>[4x]MDIKINDITLG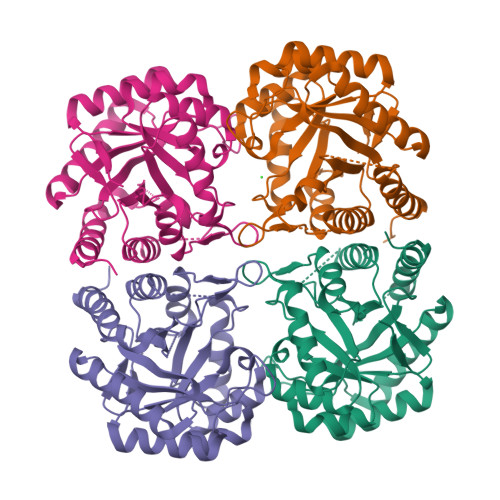NNSPFVLFGGINVLESLDSTLQTCAHYVEVTRKLGIPYIFKASFDKANRSSIHSYRGVGLEEGLKIFEKVKAEFGIPVITDVHEPHQCQPVAEVCDVIQLPAFLARQTDLVVAMAKTGNVVNIKKPQGLSPSQMKNIVEKFHEAGNGKLILCERGSSFGYDNLVVDMLGFGVMKQTCGNLPVIFDVTHSLQTRDAGSAASGGRRAQALDLALAGMATRLAGLFLESHPDPKLAKCDGPSALPLHLLEDFLIRIKALDDLIKSQPILTIE> QLEIENRIQGLHVDIEFLVRSIRQLKDEQDVFSFRYTVFSLKKTSSSDPHQSQQAQLVQATANKVDRMRKEVLDISKGLVGRLTTLVDLLLPKLDEWKVQQAASCIGAPPPELQLEQLEQWLTAGAK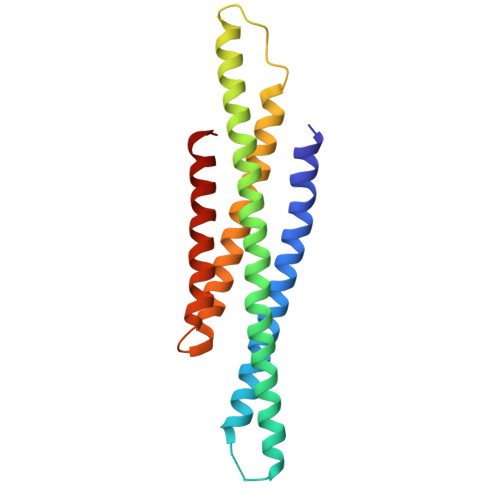FLFHLRQLLKQLKEMSHMLRYKGDMFGQGVDLQNAQVMELLQRLLQRS>GPGSFLARQLGVPQPETLRRYRAGEPPLTGSLLIGGAGRVVEPLRAALEKDYDLVGNNLGGRWADSFGGLVFDATGITEPAGLKGLHEFFTPVLRNLGRCGRVVVVGGTPEAAASTNERIAQRALEGFTRSLGKELRRGATTALVYLSPDAKPAATGLESTMRFLLSAKSAYVDGQVFSVGADDSTPPADWEKPLDGKVAIVTGAARGIGATIAEVFARDGAHVVAIDVESAAENLAETASKVGGTALWLDVTADDAVDKISEHLRDHHGGKADILVNNAGITRDKLLANMDD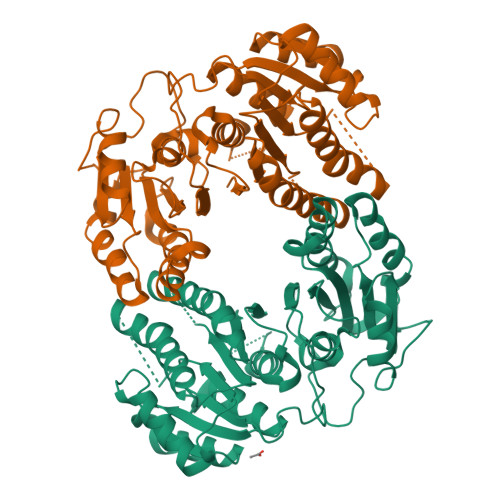ARWDAVLAVNLLAPLRLTEGLVGNGSIGEGGRVIGLSSIAGIAGNRGQTNYATTKAGMIGITQALAPGLAAKGITINAVAPGFIETQMTAAIPLATREVGRRLNSLLQGGQPVDVAEAIAYFASPASNAVTGNVIRVCG[2x]(3S,4R,5S)-3-(3-chloro-2-fluorophenyl)-4-(4-chloro-2-fluorophenyl)-4-cyano-N-[(3S)-3,4-dihydroxybutyl]-5-(2,2-dimethylpropyl)-D-prolinamide 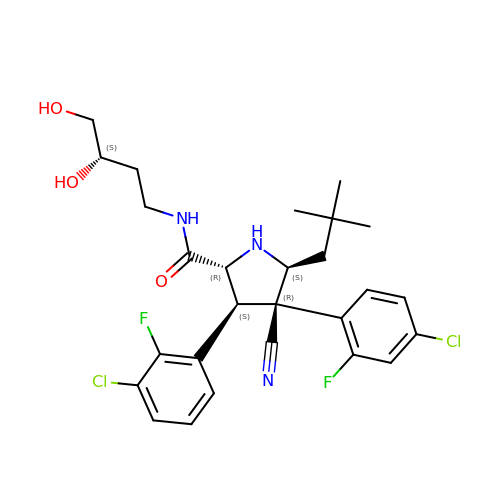| C27 H31 Cl2 F2 N3 O3 | MSOWFEGZEMCNQZ-UIHIWPSYSA-N>[2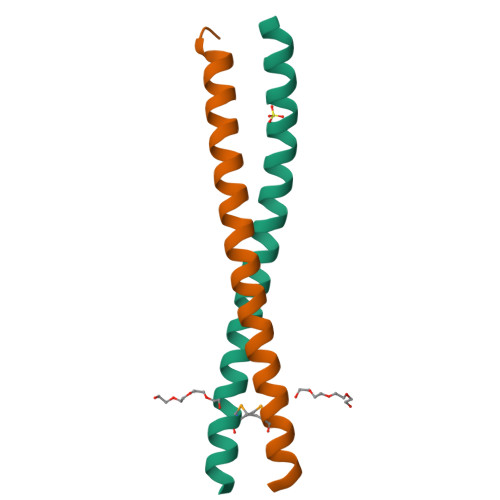x]SMLDVGNAEVKLEEENRSLKADLQKLKDELASTKQKLEKAENQVLAMRKQSEGLTKEYDRLLEEHAKL> MAAGSITT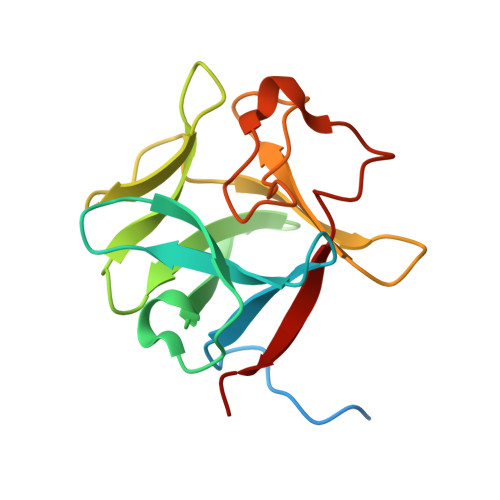LPALPEDGGSGAFPPGHFKDPKRLYCKNGGFFLRIHPDGRVDGVREKSDPHIKLQLQAEERGVVSIKGVSANRYLAMKEDGRLLASKSVTDECFFFERLESNNYNTYRSRKYTSWYVALKRTGQYKLGSKTGPGQKAILFLPMSAKS>APQQINDIVHRTITPLIEQQKIPGMAVAVIYQGKPYYFTWGYADIAKKQPVTQQTLFELGSVSKTFTGVLGGDAIARGEIKLSDPTTKYWPELTAKQWNGITLLHLATYTAGGLPLQVPDEVKSSSDLLRFYQNWQPAWAPGTQRLYANSSIGLFGALAVKPSGLSFEQAMQTRVF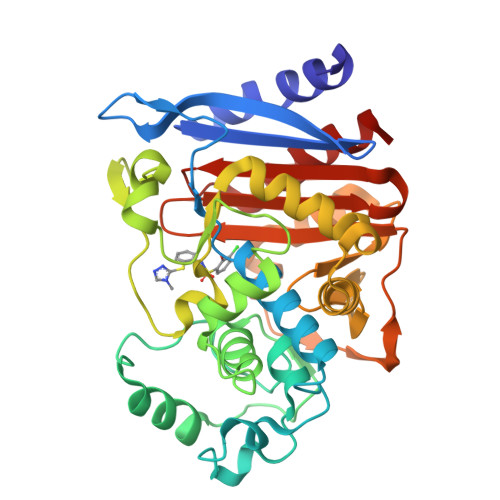QPLKLNHTWINVPPAEEKNYAWGYREGKAVHVSPGALDAEAYGVKSTIEDMARWVQSNLKPLDINEKTLQQGIQLAQSRYWQTGDMYQGLGWEMLDWPVNPDSIINGSDNKIALAARPVKAITPPTPAVRASWVHKTGATGGFGSYVAFIPEKELGIVMLANKNYPNPARVDAAWQILNALQ[2x]>[4x]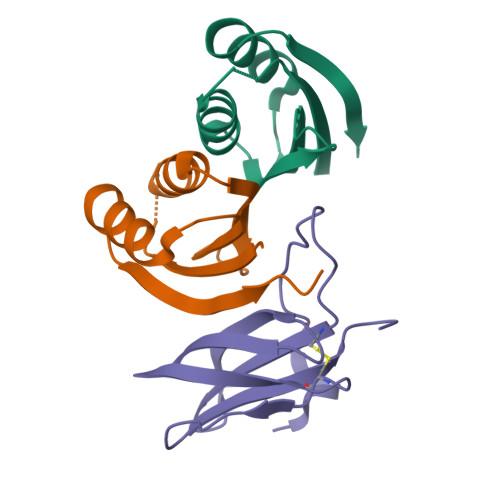GPGLKQKIVIKVAMEGNNCRSKAMALVASTGGVDSVALVGDLRDKIEVVGYGIDPIKLISALRKKVGDAELLQVEQAKED;>[2x]METGNKYIEKRAIDLSRERDPNFFDNPGIPVPECFWFMFKNNVRQDDGTCYSSWKMDMKVGPNWVHIKSDDNCNLSGDFPPGWIVLGKKRPGF>[2x]MDNFFTEGTRVWLRENGQHFPSTVNSCAEGIVVFRTDYGQVFTYKQSTITHQKVTAMHPTNEEGVDDMASLTELHGGSIMYNLFQRYKRNQIYTYIGSILASVNPYQPIAGLYEPATMEQYSRRHLGELPPHIFAIANECYRCLWKRHDNQCILISGESGAGKTESTKLILKFLSVISQQSLELSLKEKTSCVERAILESSPIMEAFGNAKTVYNNNSSRFGKFVQLNICQKGNIQGGRIVDYLLEKNRVVRQNPGERNYHI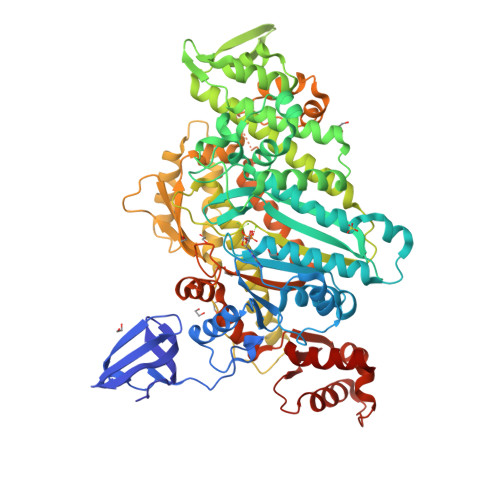FYALLAGLEHEEREEFYLSTPENYHYLNQSGCVEDKTISDQESFREVITAMDVMQFSKEEVREVSRLLAGILHLGNIEFITAGGAQVSFKTALGRSAELLGLDPTQLTDALTQRSMFLRGEEILTPLNVQQAVDSRDSLAMALYACCFEWVIKKINSRIKGNEDFKSIGILDIFGFENFEVNHFEQFNINYANEKLQEYFNKHIFSLEQLEYSREGLVWEDIDWIDNGECLDLIEKKLGLLALINEESHFPQATDSTLLEKLHSQHANNHFYVKPRVAVNNFGVKHYAGEVQYDVRGILEKNRDTFRDDLLNLLRESRFDFIYDLFEHVSSRNNQDTLKCGSKHRRPTVSSQFKDSLHSLMATLSSSNPFFVRCIKPNMQKMPDQFDQAVVLNQLRYSGMLETVRIRKAGYAVRRPFQDFYKRYKVLMRNLALPEDVRGKCTSLLQLYDASNSEWQLGKTKVFLRESLEQKLEKRREEE> MGLLLLVLILTPSLAAYRHPDFPLLEKAQQLLQSTGSPYSTNCWLCTSSSTETPGTAYPASPREWTSIEAELHISYRWDPNLKGLMRPANSLLSTVKQDFPDIRQKPPIFGPIFTNINLMGIAPICVTAKRKNGTNVGTLPSTVCNVTFTVDPNQQTYQTYTHNQFRHQPRFPKPPNITFPQGTLLDKSTRFCQGRPSSCSTRNFWFRPADYNQCLQISNLSSTAEWVLLDQTRNSLFWENKTKGANQSQTPCVQVLAGMTIATSYLGISAVSEFFGTSLTPLFHFHISTCLKTQGAFYICGQSIHQCLPSNWTGTCTIGYVTPDIFIAPGNLSLPIPIYGNSPLPRVRRAIHFIPLLAGLGILAGTGTGIAGITKASLTYSQLSKEIANNIDT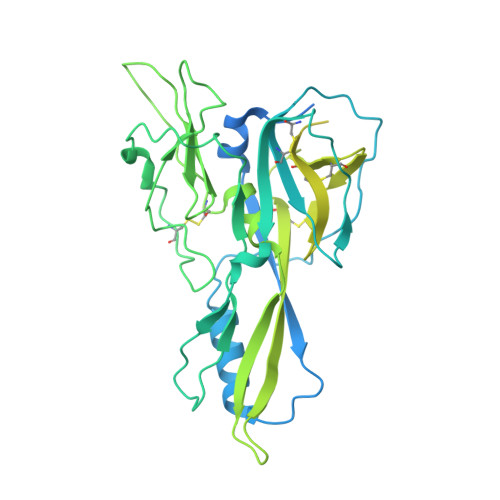MAKALTTMQEQIDSLAAVVLQNRRGLDMLTAAQGGICLALDEKCCFWVNQSGKVQDNIRQLLNQASSLRERATQGWLNWEGTWKWFSWVLPFIGPLVSLLLLLLFGPCLLNLITQFVSSRLQAIKLQTNLSAGRHPRNIQESPF> MNRSVNIAKNLIQTYRAMSVQSRFAFSTREEEWLDKRTKSQEKVYFDQEDRKA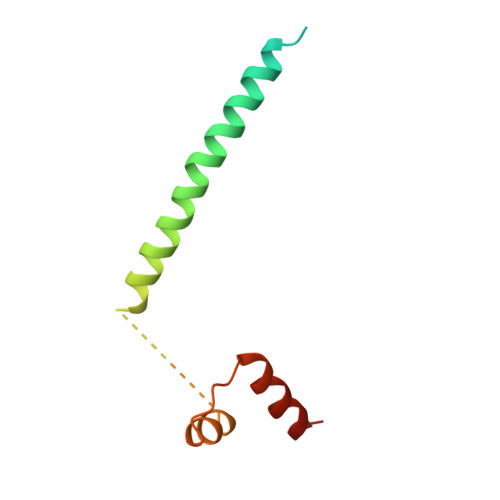MKRLLEKLNTTSKFVEDSEYLAPQNLEVENILKRYHINYTQALIDELVDWKTGKN> MSVETPSALADSSPHTAPGSAGRSLELGAADIQDLESFEAGRGALPARAYLQSDAPRLSLNGEWQFRLSPGSRVAPDDGWQLGEALNGFESLPVPSSWPMHGHGAPAYTNVQFPFAVEPPHVPEANPIGDHLVVFEAGPEFFPHALLRFDGIESAGTVWLNGVELGTTRGSRLAHEFDVSGILEQGENTLAVRVAQFSAASYVEDQAMWWLPGIFRDVTLQARPAAGIDDVFVHAGYDHITGEGILKVEASRGGQAIDAVVRVPELALELAAGTEVRVPAVEPWSAEVPKLYEAAVSAAGESVALQIGFRSIAIEDAQFKVNGRRILLRGVNRHEHHPRLGRVVPRDVVEAELRLMKQHNINAIRTSHYPPHPQFLALADQLGFYVVLECDLETHGFESAGWAQNPSDDPQWEDALVDRMRRTVERDKNHASVVMWSLGNEAGTGRNLAAMSRWTKDRDPSRPIHYEGDWSSEHVDVYSRMYASQAETALIGQGIEPALNDAALDARRRAMPFVLCEYVHAMGNGPGGMSEYQALFEKYPRLMGGFVWEWLEHGITVSTADGVDHYGYGGDFGEEVHDGNFVTDGLVDADRRPRPGLLDFKKVIEPLRIDVARDWTGFTLRNGQDFADTSAFSFRYEVEADGGALDGGTVDVAPVAPQSETVVELPGSVAALAAGLSDGRPAVLTVRAVLGADSAWADAGHEVAWGQSVREPGAPVPPAPVEPVQVQDSELTLGPVVFSRATGMPTSIGGVPVEKLGLTLWWAPTDNDLGREWGGADERPLATQWKDAGLNRLHTRLLGISANPGQDGGETLTVRTRVSAADKQYGVLVDYTWSTDGETVGLRTQVRRDGTWVNRGFEVEWARIGLEFVLGEETELVSWFGQGPHQSYPDTGQGARAGWFSLPLAKMDVEYVRPQECGARSGSRSAALQLGGRTLEICGDPFALTVRPYSQDVLDAAAHRPDLKADGRTYLYVDHALRGVGTAACGPGVLEQYRLKPRDADFILTLKVRS

Psychrophilic β-d-galactosidase from Arthrobacter sp. 32cB is an interesting candidate for industrial use, as it can hydrolyze lactose at rate comparable to mesophilic βDG from Kluyveromyces lactis. Furthermore, it exhibits additional transglycosylation activity, it catalyzes synthesis of GOS and HOS, for example: lactulose and alkyl glycosides. The functional dimer of ArthβDG has two independent active sites. Each of them is located on the top of TIM-barrel Domain 3 and is constituted of residues from both subunits of the dimer.

The ArthβDG_E517Q exhibited no catalytic activity, whereas activity of mutant ArthβDG_D207A was severely depleted. The mutation of the residue involved in the stabilization of galactosyl moiety within active site, D207, diminished the enzyme’s activity. Results of the TSA (thermofluor shift assay) of ArthβDG_D207A did not exhibit significant differences compared with ones obtained for wild-type protein ArthβDG. The structures of ArthβDG mutants: ArthβDG_D207A and ArthβDG_E517Q, were solved proving that the point mutations within the active site of ArthβDG have no destabilizing effect on protein’s structure. In the case of mutant ArthβDG_D207A, where a larger side chain was substituted with alanine residue, the change in active site size and shape was introduced. Especially surprising was the gravity of mutation of D207 to alanine, which is part of Domain 1. It is situated on the top of a part of Domain 1, which inserts itself in a space between the top of Domain 3 TIM-barrel and highly flexible C-terminal region of Domain 3, and constitutes bottom of the active site, which means that its mutation to alanine has a significant impact on active site volume. As such, not only a stabilizing interaction between D207 and O4 hydroxyl of galactosyl moiety is lost but also the transfer of substrate from shallow to deep binding site of the enzyme is disrupted.>[2x]SNEYDEYIANHTDPVKAINWNVIPDEKDLEVWDRLTGNFWLPEK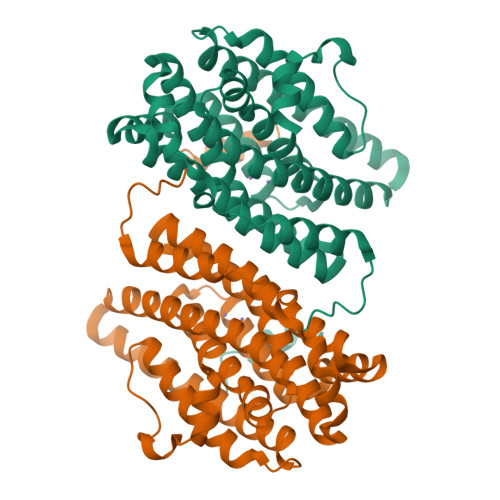IPVSNDIQSWNKMTPQEQLATMRVFTGLTLLDTIQGTVGAISLLPDAETMHEEAVYTNIAFMESVHAKSYSNIFMTLASTPQINEAFRWSEENENLQRKAKIIMSYYNGDDPLKKKVASTLLESFLFYSGFYLPMYLSSRAKLTNTADIIRLIIRDESVHGYYIGYKYQQGVKKLSEAEQEEYKAYTFDLMYDLYENEIEYTEDIYDDLGWTEDVKRFLRYNANKALNNLGYEGLFPTDETKVSPAILSSLS> GSTLQPLENSTRQEKLLYPKLNQLSNSINAAVAFLLEARNLEGWWQDFNFPQAASI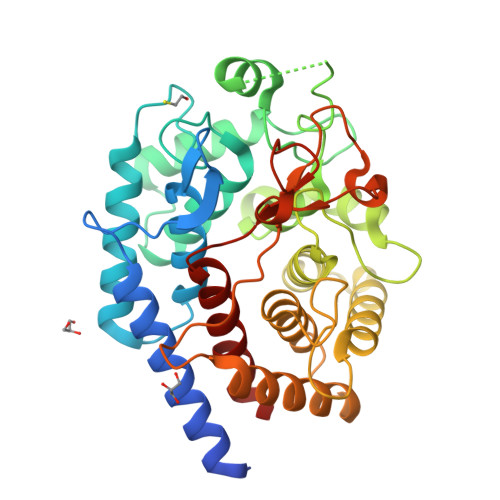GDEWVTAYVGTMLATLPYAHVHEALMQAWELLKIRDHRPTGEWGYNYILCGDADTTGWALQLAAAVGASDSERAQQARAALATHLQPNGGIATFAEESIRAFIKVPDLANVSFQGWCGAHTCVSAAVAALPEFRSRLHDYLRVTQTSQGNWEGYWWSDHEYTTALTAEALAAGGQAADQPSIEQAVAWGLKRLCPQGFVATSKHPNGSTFATAWCLRLLLLNTVDAEVKAARAAAIGWLLEQQRPNGSWVSSAYLRIPYPFDRNPNQFPHWRYYDEIEGDKRFEGSIIFDHNSIFTTATVVNSLVKAAPML>[2x]MTRILTAFKVVRTLKTGFGFTNVTAHQKWKFSRPGIRLLSVKAQTAHIVLEDGTKMKGYSFGHPSSVAGEVVFNTGLGGYPEAITDPAYKGQILTMANPIIGNGGAPDTTALDELGLSKYLESNGIKVSGLLVLDYSKDYNHWLATKSLGQWLQEEKVPAIYGVDTRMLTKIIRDKGTMLGKIEFEGQPVDFVDPNKQNLIAEVSTKDVKVYGKGNPTKVVAVDCGIKNNVIRLLVKRGAEVHLVPWNHDFTKMEYDGILIAGGPGNPALAEPLIQNVRKILESDRKEPLFGISTGNLITGLAAGAKTYKMSMANRGQNQPVLNITNKQAFITAQNHGYALDNTLPAGWKPLFVNVNDQTNEGIMHESKPFFAVQFHPEVTPGPIDTEYLFDSFFSLIKKGKATTITSVLPKPALVASRVEVSKVLILGSGGLSIGQAGEFDYSGSQAVKAMKEENVKTVLMNPNIASVQTNEVGLKQADTVYFLPITPQFVTEVIKAEQPDGLILGMGGQTALNCGVELFKRGVLKEYGVKVLGTSVESIMATEDRQLFSDKLNEINEKIAPSFAVESIEDALKAADTIGYPVMIRSAYALGGLGSGICPNRETLMDLSTKAFAMTNQILVEKSVTGWKEIEYEVVRDADDNCVTVCNMENVDAMGVHTGDSVVVAPAQTLSNAEF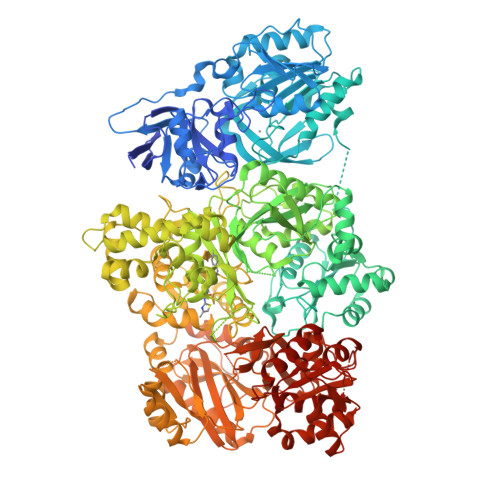QMLRRTSINVVRHLGIVGECNIQFALHPTSMEYCIIEVNARLSRSSALASKATGYPLAFIAAKIALGIPLPEIKNVVSGKTSACFEPSLDYMVTKIPRWDLDRFHGTSSRIGSSMKSVGEVMAIGRTFEESFQKALRMCHPSIEGFTPRLPMNKEWPSNLDLRKELSEPSSTRIYAIAKAIDDNMSLDEIEKLTYIDKWFLYKMRDILNMEKTLKGLNSESMTEETLKRAKEIGFSDKQISKCLGLTEAQTRELRLKKNIHPWVKQIDTLAAEYPSVTNYLYVTYNGQEHDVNFDDHGMMVLGCGPYHIGSSVEFDWCAVSSIRTLRQLGKKTVVVNCNPETVSTDFDECDKLYFEELSLERILDIYHQEACGGCIISVGGQIPNNLAVPLYKNGVKIMGTSPLQIDRAEDRSIFSAVLDELKVAQAPWKAVNTLNEALEFAKSVDYPCLLRPSYVLSGSAMNVVFSEDEMKKFLEEATRVSQEHPVVLTKFVEGAREVEMDAVGKDGRVISHAISEHVEDAGVHSGDATLMLPTQTISQGAIEKVKDATRKIAKAFAISGPFNVQFLVKGNDVLVIECNLRASRSFPFVSKTLGVDFIDVATKVMIGENVDEKHLPTLDHPIIPADYVAIKAPMFSWPRLRDADPILRCEMASTGEVACFGEGIHTAFLKAMLSTGFKIPQKGILIGIQQSFRPRFLGVAEQLHNEGFKLFATEATSDWLNANNVPATPVAWPSQEGQNPSLSSIRKLIRDGSIDLVINLPNNNTKFVHDNYVIRRTAVDSGIPLLTNFQVTKLFAEAVQKSRKVDSKSLFHYRQYSAGKAA> QSEARRRILETAWRLIARRGYHNVRIHDIASELGTSNATIHYHFPSKKDILLEALRRNVKLAFDRQVAELHTIADARERLVRLVELQLPTPGLLRDEWSVWLQVWTESTLNPKIRDLYNDAYDRWYQTIAMTIRTGQKQGVFRDQDADELATRLSALIDGLGIQVLTGKR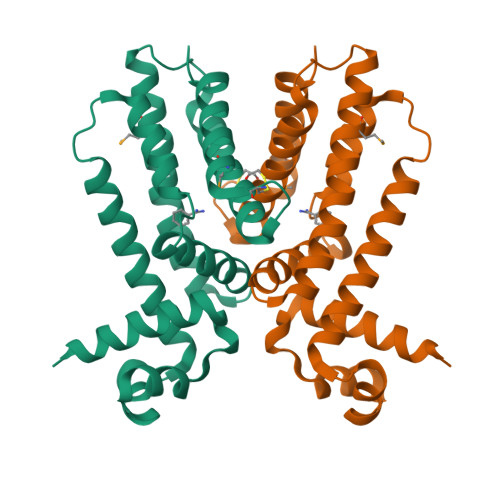GCSVDHMRQHLNDFIEHNIVERRP Like DsbC, PmScsC is a protein disulfide isomerase with a thioredoxin-fold catalytic domain, redox-active cysteines and a redox-partner membrane protein (PmScsB) that reduces the active-site cysteines. Unlike DsbC, PmScsC is trimeric rather than dimeric. The native PmScsC protomer consists of an N-terminal trimerization stem with an 11-amino-acid flexible linker connected to a C-terminal thioredoxin-fold catalytic domain harbouring a CXXC active site. The region responsible for this conformational flexibility is an 11-amino-acid linker within the trimerization stem of the protein.

PmScsCΔN lacks the first 41 amino acids of the native PmScsC construct; its loss of disulfide isomerase activity and gain of dithiol oxidase activity has been reported previously. The crystal structure of PmScsCΔN reveals, as expected, a monomeric protein that closely resembles the catalytic domain from the full-length PmScsC protomer. Crystals of the PmScsCΔN mutant diffracted to a resolution of 2.15 Å at the Australian Synchrotron. The X-ray crystal structure of PmScsCΔN agrees with previous MALS data showing that this variant is monomeric. The crystal structure is also consistent with solution SAXS data and the low-resolution model obtained from SAXS analysis. Although the PmScsCΔN crystal structure is very similar to the structures of the catalytic domains in each of the three crystal structures of native PmScsC, unlike the native enzyme it lacks disulfide isomerase (disulfide-shuffling) activity and instead has dithiol oxidase (disulfide-forming) activity. The PmScsC catalytic domain has an acidic catalytic cysteine and an energetically unfavourable disulfide, which are also features of the archetypal but monomeric dithiol oxidase EcDsbA, so it is perhaps not surprising that the removal of the N-terminal trimerization residues leads to oxidase activity in a model assay. Moreover, the structural similarity between monomeric PmScsCΔN and the catalytic domains of native trimeric PmScsC supports the notion that it is the N-terminal stem, which defines whether the catalytic domain is monomeric or trimeric, that is the determinant of isomerase or oxidase activity. In the crystal packing, PmScsCΔN makes contact with six symmetry-related molecules, but none involve packing against the catalytic motif or the positively charged surface patch that surrounds it. In the crystal packing of the PmScsCΔN structure (which does not have the constraint of the trimerization stem), there are no contacts involving the positively charged surface patch near the catalytic motif, suggesting that packing against this site is not favoured.

> SNAQFRQALASEHDALYNDAASPRIGAKDAKLVLVSFTDYNCPYCKRFDPLLEKITEQYPDVAVIIKPLPFKGESSAKASQAVLSVWKEDPKAFLALHQRLMQKKTMLDNASIEDAMKSTNTSKIKLTDDSLKTLQNNLELSRKLGIQGTPATVIGDTILPGAVDYDQLEIIVKEQLAKVKK>HY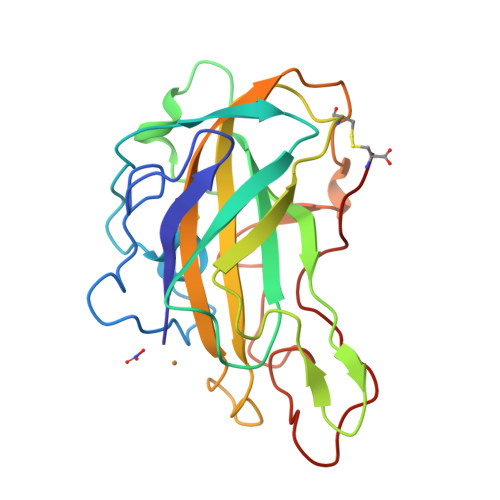TFPKVWANSGTTADWQYVRRADNWQNNGFVDNVNSQQIRCFQSTHSPAQSTLSVAAGTTITYGAAPSVYHPGPMQFYLARVPDGQDINSWTGEGAVWFKIYHEQPTFGSQLTWSSNGKSSFPVKIPSCIKSGSYLLRAEHIGLHVAQSSGAAQFYISCAQLSITGGGSTEPGANYKVSFPGAYKASDPGILININYPVPTSYKNPGPSVFTC[2x]> IVGGTNSSWGEWPWQVSLQVKLTAQRHLCGGSLIGHQWVLTAAHCFDGLPLQDVWRIYSGILNLSDITKDTPFSQIKEIIIHQNYKVSEGNHDI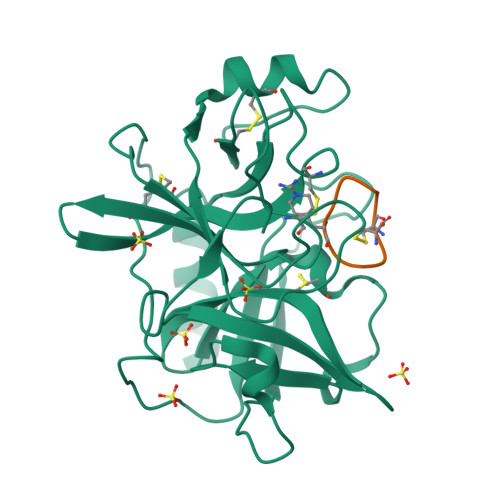ALIKLQAPLNYTEFQKPISLPSKGDTSTIYTNCWVTGWGFSKEKGEIQNILQKVNIPLVTNEECQKRYQDYKITQRMVCAGYKEGGKDACKGDSGGPLVCKHNGMWRLVGITSWGEGCARREQPGVYTKVAEYMDWILEKTQSSD;> CPARFAALFC1-PYRIDIN-3-YLBUTAN-1-ONE | C9 H11 N O | 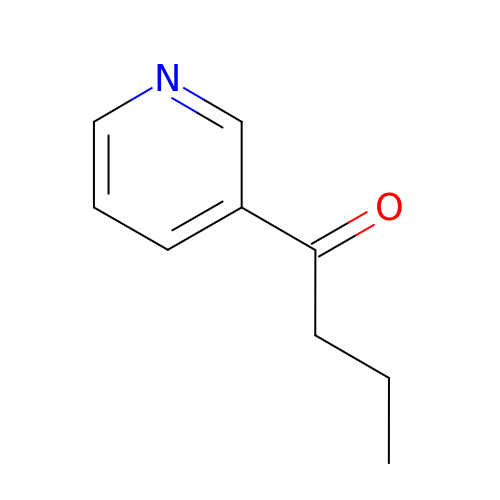JORUAYHMUWRFNM-UHFFFAOYSA-N> MFAWWGRTVYQFRYIVIGVMVALCLGGGVYGISLGNHVTQSGFYDEGSQSVAASLIGDEVYGRDRTSHVVAILTPPDDKKVTDKAWQKKVTEELDQVVKDHEDQIVGWVGWLKAPDTTDPTVSAMKTQDLRHTFISIPLQGDDDDEILKNYQVVEPELQQVNGGDIRLAGLNPLASELTGTIGEDQKRAEVAAIPLVAVVLFFVFGTVIAAALPAIIGGLAIAGALGIMRLVAEFTPVHFFAQPVVTLIGLGIAIDYGLFIVSRFREEIAEGYDTEAAVRRTVMTSGRTVVFSAVIIVASSVPLLLFPQGFLKSITYAIIASVMLAAILSITVLAAALAILGPRVDALGVTTLLKIPFLANWQFSRRIIDWFAEKTQKTKTREEVERGFWGRLVNVVMKRPIAFAAPIL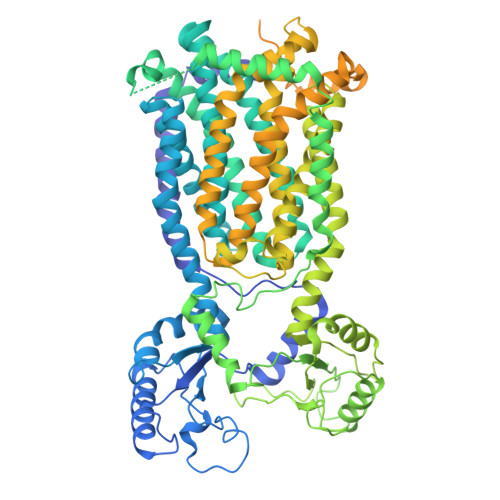VVMVLLIIPLGQLSLGGISEKYLPPDNAVRQSQEQFDKLFPGFRTEPLTLVMKREDGEPITDAQIADMRAKALTVSGFTDPDNDPEKMWKERPANDSGSKDPSVRVIQNGLENRNDAAKKIDELRALQPPHGIEVFVGGTPALEQDSIHSLFDKLPLMALILIVTTTVLMFLAFGSVVLPIKAALMSALTLGSTMGILTWMFVDGHGSGLMNYTPQPLMAPMIGLIIAVIWGLSTDYEVFLVSRMVEARERGMSTAEAIRIGTATTGRLITGAALILAVVAGAFVFSDLVMMKYLAFGLLIALLLDATIIRMFLVPAVMKLLGDDCWWAPRWMKRVQEKLGLGETELPDERKRPTVRESETDQRALVGVGAPPPPPRPHDPTHPAPEPVRPMPPMRSNAPSAAGTARISTPPQPPQPPQAPAQQAGDEPATTRFAMARNAVRNAVNSAVHGGAGSAAAPTERAPRPGGPAQPPAPPQREEREIESWLGALRGPAPAKNVPQPPAQPQRPSTDTTRAMPPQGRPPAGPADRGNENAPTTAFSAQRPPNGGAPADATTAIPTPPQREQEPSTEKLNTREDAPEDPETKRRGGGMSAQDLLRREGRL> DSISLSLINEGPS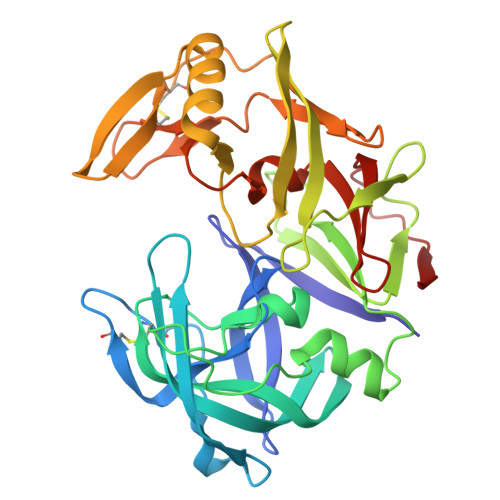YASKVSVGSNKQQQTVIIDTGSSDFWVVDSNAQCGKGVDCKSSGTFTPSSSSSYKNLGAAFTIRYGDGSTSQGTWGKDTVTINGVSITGQQIADVTQTSVDQGILGIGYTSNEAVYDTSGRQTTPNYDNVPVTLKKQGKIRTNAYSLYLNSPSAETGTIIFGGVDNAKYSGKLVAEQVTSSQALTISLASVNLKGSSFSFGDGALLDSGTTLTYFPSDFAAQLADKAGARLVQVARDQYLYFIDCNTDTSGTTVFNFGNGAKITVPNTEYVYQNGDGTCLWGIQPSDDTILGDNFLRHAYLLYNLDANTISIAQVKYTTDSSISAV> MPQFTAGNSHVAQNRRNYMDPSYKLEKLRDIPEEDIVRLLAHRAPGEEYKSIHPPLEEMEEPDCAVRQIVKPTEGAAAGDRIRYVQYTDSMFFSPITPYQRAWEALNRYKGVDPGVLSGRTIIEARERDIEKIAKIEVDCELYDTARTGLRGRTVHGHAVRLDKDGMMFDALRRWSRGADGTVTYVKDMIGGAMDKEVTLGKPLSDAELLKKTTMYRNAQGGVWQEADDPES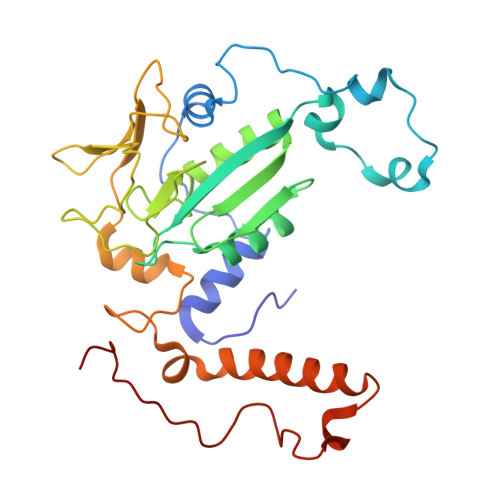MDVTAQIHWKRSVGGFQPWAKMKDIKGGKKDVGVKNLKLFTPRGGVE> MDFKYSRELKLESLDALNLTEGIPLRVNENIDLEFRGIERAHSDWERYVGKLNGFHGGRGPQFGFVSACIPECL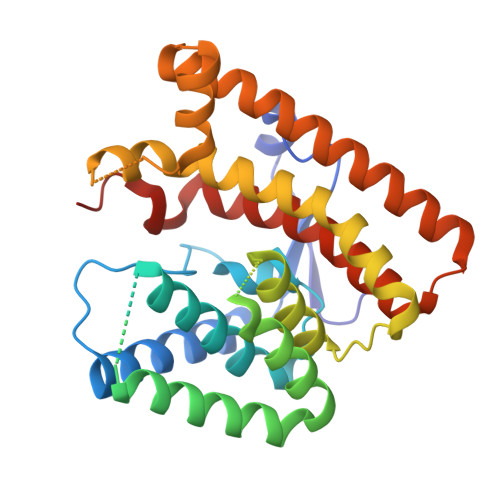PERMETVSYANEFAFLHDDMTDAASKDQVNGLNDDLLGGLDFTTEARSSASGKQQMQAKLLLEMLSIDRERTMVTIKAWADFMRGAAGRDHHRGFSSLDEYIPYRCADCGEKFWFGLVTFAMALSIPEQELELVQRLAQNAYLAAGLTNDLYSYEKEQLVAERSGTGQVFNAIAVIMQEHSVSISEAEDICRGRIREYAAKYVRDVADLRAKNELSRDSLAYLETGLYGISGSTAWNLDCPRYQVSTFVDFKTP>[2x]MSSIKVECVLRENYRCGESPVWEEASQSLLFVDIP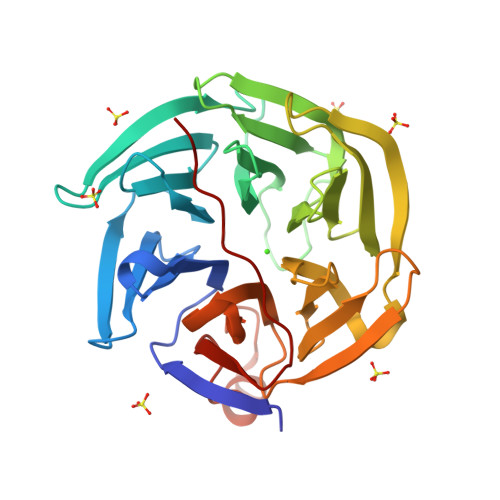SKIICRWDTVSNQVQRVAVDAPVSSVALRQLGGYVATIGTKFCALNWENQSVFVLAMVDEDKKNNRFNDGKVDPAGRYFAGTMAEETAPAVLERHQGSLYSLFPDHSVKKYFDQVDISNGLDWSLDHKIFYYIDSLSYTVDAFDYDLQTGQISNRRIVYKMEKDEQIPDGMCIDAEGKLWVACYNGGRVIRLDPETGKRLQTVKLPVDKTTSCCFGGKDYSEMYVTCARDGLNAEGLLRQPDAGNIFKITGLGVKGIAPYSYAG O-glycosylation of the protein CST1 by the mucin-type O-glycosyltransferase T. gondii (Txg) GalNAc-T3 influences cyst wall rigidity and stability. The strict glycopeptide-preferring enzyme TxgGalNAc-T3 then adds GalNAc to acceptor Thr one position N-terminal to existing Thr-O-GalNAcs and is predicted to sequentially O-glycosylate Thr rich repeats within the mucin domain of CST1. The structures reveal a unique GalNAc binding pocket that dictates the substrate preference of TxgGalNAc-T3, which is coupled to a 2nd metal binding site that is strictly conserved among apicomplexan homologs.

To investigate the basis of the substrate specificity and function of TxgGalNAc-T3, we solved the x-ray co-crystal structures of TxgGalNAc-T3 in complex with Mn2+, a non-hydrolysable form of UDP-GalNAc (UDP-2-(acetylamino)−4-F-D-galactosamine disodium salt, UDP-GalNAc-F) and each of the following glycopeptides: CST1.4, Muc5AC-3,13, Muc5AC-3, Muc5AC-13, and SRS13.2 from 2.2-2.9 Å resolution. The catalytic domain adopts the conserved GT-A fold and the active site contains a DXH motif (Asp276, Ser277, His278), where Asp276, His278, His414, UDP, and a water molecule coordinate Mn2+A with octahedral geometry. Although the glycopeptide amino acid sequences vary, both CST1.4 and Muc5AC-3,13 are similarly bound along the active site substrate groove with the acceptor Thr positioned for catalysis, adopting a similar conformation seen in peptides bound to metazoan GalNAc-Ts. Thr-O-GalNAc at the +1 position on the glycopeptides is bound to a pocket in TxgGalNAc-T3 consisting of His333 (catalytic domain) and Glu554 (lectin domain) that interact with GalNAc via sidechain H-bonds, and Ser334 (catalytic domain), which interacts with GalNAc through a mainchain H-bond. Mn2+N is coupled to the GalNAc binding pocket through coordination to His333 and indirect coordination to Glu554 via water. Poor electron density for the remaining unmodeled residues in CST1.4 and Muc5AC-3,13 suggests that they are disordered in the structure and making transient interactions with TxgGalNAc-T3. Loop II flexibility and the interaction that occurs between the Gly319 backbone carbonyl and an amide group on both di-glycopeptide substrates (Muc5AC-3,13 and CST1.4) allows TxgGalNAc-T3 to accommodate and modify substrates with variable sequences. Thus, a role for the lectin domain in activity enhancement through interactions with a distal GalNAc on a di-glycopeptide has not been shown but is consistent with the lack of electron density at the C-terminal Thr-O-GalNAc in the co-crystal structures of TxgGalNAc-T3 bound to the di-glycopeptides CST1.4 and Muc5AC-3,13.

> GARDVQEGVSSFEESGGAQLPPRVHALEVLEGAGPGRLHGRLGIKPDGQPGYTRAPSPPTDLSMPQALARGGGFNLYLSDHLELDRTAPDARHASCRQLHYDLSTLPKASVIIVFYNEPFSTLMRSVHSVLNGTPPQILEELILVDDGSTLPYIREDGNQQLVEYLKLLPAKVRLIRNEVRKGIVGARMKGIRASRAPIFAILDSHIEVSPQWLEPLLLRIKEDSRRVVMPQIDGIDAETFKHIAGGIGCKLGFLWKLMEHSYEGHQTARLPPEERQPSPTDFQTSPAMAGGLFAANKAFFFDVGAYDEDFQFWGTENLELSFRLWQCGGVLECAPCSRVYHIFRKGGSGYSSPGDSITINKMRTMLWMDEYADLAWRVIGKPRVNYRPESLEKRREWRKRKGCKSFRWFMENVFPEGDVVTLDDVPYLGPLRNDKIGMCLDNMGWASPGHAVGLEYCHGGDTQTFMFFRKVGHVMPVNDDEACLQPSGRLDWCRGTAQFWWDFTSSGQLMFRETKQCLSAFGRKLRMVECDDTDPYQIWSWTAYNPPDTFTFPSVSRSIRSG;> TTTTKKPTTTTTTTKKP>[2x]MASMTGGQQMGRDEAGITGTWYNQLGSTFIVTAGA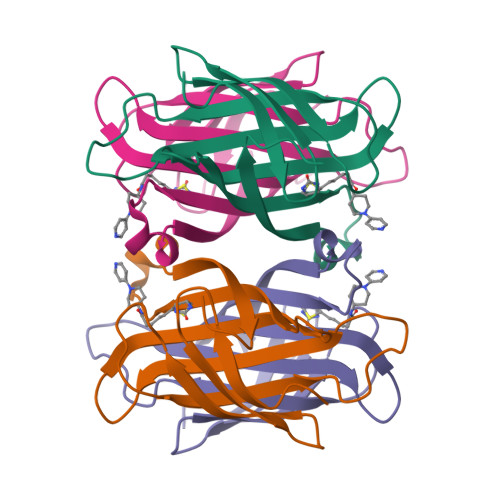DGALTGTYESAAGKAESRYVLTGRYDSAPATDGSGTALGWTVAWKNNYRNAHSATTWSGQYVGGAEARINTQWLLTMGATEANGWASTLVGHDTFTKVKPSAASIDAAKKAGVNNGNPLDAVQQ>[2x]GEQAQQARELGQSLAQEVKAATERLSLGSRDVAERLRLSKDIGRLIEAVETSV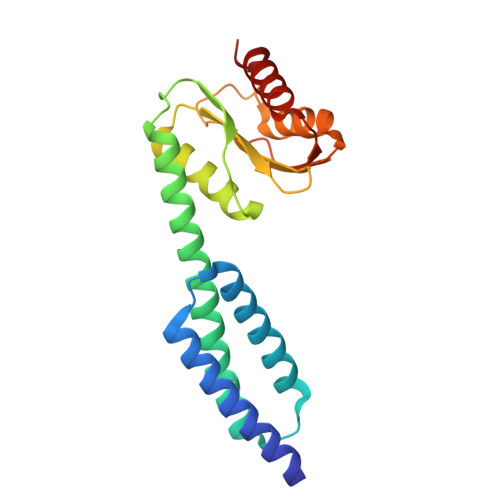MPQWQRRELLATVKMLQRRANTAIRKLQMGQAAKKTQELLERHSKGPLIVDTVSAESLSVLVKVVRQLCEQAPSTSVLLLSPQPMGKVLCACQVAQGAMPTFTAEAWALAVCSHMGGKAWGSRVVAQGTGSTTDLEAALSIAQTYALSQLL R-1,2-PROPANEDIOL | 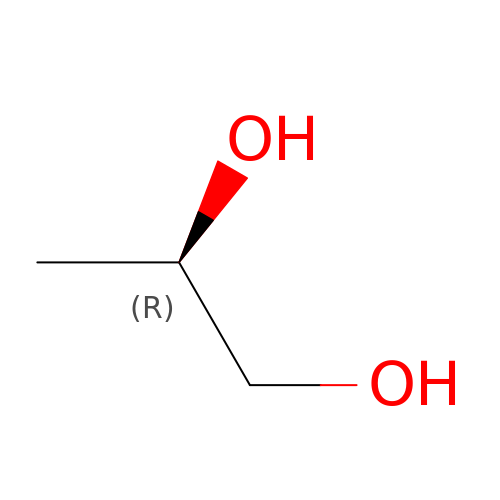C3 H8 O2 | DNIAPMSPPWPWGF-GSVOUGTGSA-N> MNTDAIESMVRDVLSRMNSLQGEAPAAAPAAGGASRSARVSDYPLANKHPEWVKTATNKTLDDFTLENVLSNKVTAQDMRITPETLRLQASIAKDAGRDRLAMNFERAAELTAVPDDRILEIYNALRPYRSTKEELLAIADDLESRYQAKICAAFVREAATL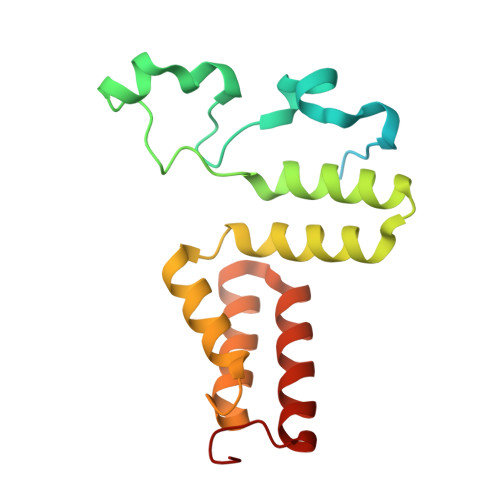YVERKKLKGDD>SNAMPLPKSLKYGDTIGIYSPSSPVTYTSPKRFERAKSYLLQKGFHILEGSLTGRYDYYRSGSIQERAKELNALIRNPNVSCIMSTIGGMNSNSLLPYIDYDAFQNNPKIMIGYSDATALLLGIYAKTGIPTFYGPALVPSFGEFEPFVDDTYKYFLETLLHDQALPYNIKQPLFWSDEFINWEEKTKEKELRPNNWISVTNGQATGRVIGGNLNTIQGIWGSPYMPCIQEGDILFIEDSRKDAATIERSFSFLKINGVFDKVSGIILGKHEQFDDCGTNRKPYEILLEVLQNQRIPLLADFDCCHTH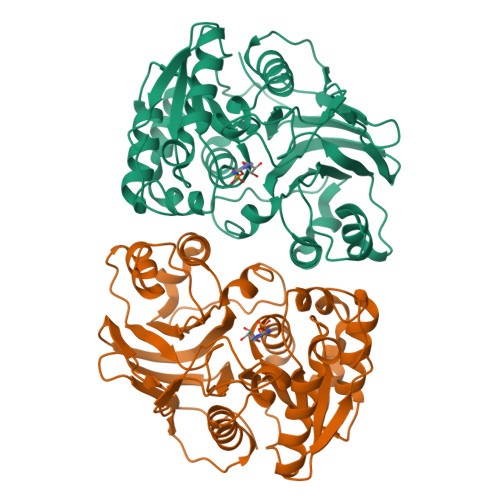PMITMPIGVQVKMDATNKTIHILEKWKI[2x]> MRAEDLPKAVVFLEPQWYRVLEKDSVTLKCQGAYSPEDQSTRWFHNESLISSQTSSYFIAAARVNNSGEYRCQTSLSTLSDPVQLEVHIGWLLLQAPRWVFKEEESIHLRCHSWKNTLLHKVTYLQNGKGRKYFHQNSDFYIPKATLKDSGSYFCRGLIGSKNVSSETVQIT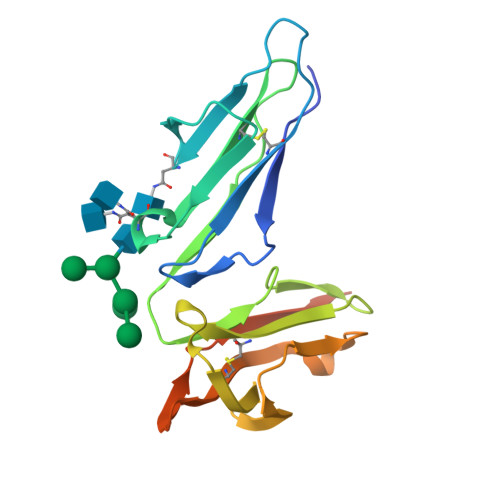ITQDLAVSSISSFFPPGYQV> GPHMSTEKAPAALGPYSQAIKANNLVFLSGVLGLIPETGKFVSESVEDQTEQVLKNMGEILKASGADYSSVVKTTIMLADLADFKTVNEIYAKYFPAPSPARSTYQVAALPLNAKIEIECIATL

Arabidopsis thaliana RidA (AtRidA) is targeted to chloroplasts. By converting the reactive enamine/imines to harmless 2-oxoacids, RidA preempts damage to BCAT3 and ensures that the isoleucine biosynthesis can proceed. In this study, we determined the crystal structures of apo-AtRidA and its complex with pyruvate, and analyzed its structural basis for ligand recognition. The RidA domain retains the basic overall fold, and also preserves the homotrimeric structure with the characteristic interfacial clefts.

The current crystal structure was produced by the construct starting from S68 (named AtRidA-S68), and it diffracted to a resolution of 2.0 Å. In the final model, residues S80-L187, as well as 85 water molecules are resolved. Each asymmetric unit contains a single monomer, with a Matthew’s coefficient of 1.85 and an estimated solvent content of 33.7%. The model shows a mixed β-sheet packed against two long α-helices. In the β-sheet, the strands are antiparallel except for the outermost strand β4, which is parallel to β3. An extended loop L91-E110 is located between β2 and α1. AtRidA-S68 crystal structure is disordered in the first 12 residues, which accounts for the missing strand. The space group of apo-AtRidA is H3 and through symmetry operation, a homotrimer can be generated. There is a central cavity in the barrel-like trimeric structure, whose height is ~31 Å. The buried surface between the neighboring monomers is 1306.2 Å2.> MSSAIKEVQGAPVKWVTNWTPEAIRGLVDQEKGLLDPRIYADQSLYELELERVFGRSWLLLGHESHVPETGDFLATYMGEDPVVMVRQKDKSIKVFLNQCRHRGMRICRSDAGNAKAFTCSYHGWAYDIAGKLVNVPFEKEAFCDKKEGDCGFDKAEWGPLQARVATYKGLVFANWDVQAP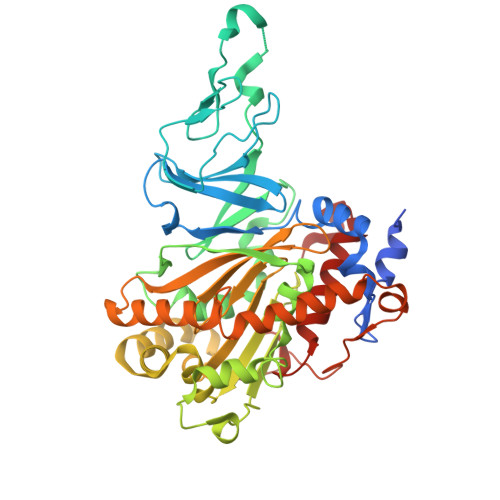DLETYLGDARPYMDVMLDRTPAGTVAIGGMQKWVIPCNWKFAAEQFCSDMYHAGTTTHLSGILAGIPPEMDLSQAQIPTKGNQFRAAWGGHGSGWYVDEPGSLLAVMGPKVTQYWTEGPAAELAEQRLGHTGMPVRRMVGQHMTIFPTCSFLPAMNNIRIWHPRGPNEIEVWAFTLVDADAPAEIKEEYRRHNIRNFSAGGVFEQDDGENWVEIQKGLRGYKAKSQPLNAQMGLGRSQTGHPDFPGNVGYVYAEEAARGMYHHWMRMMSEPSWATLKP> IVGGTDATLGEFPYQLSFQETFIGFSF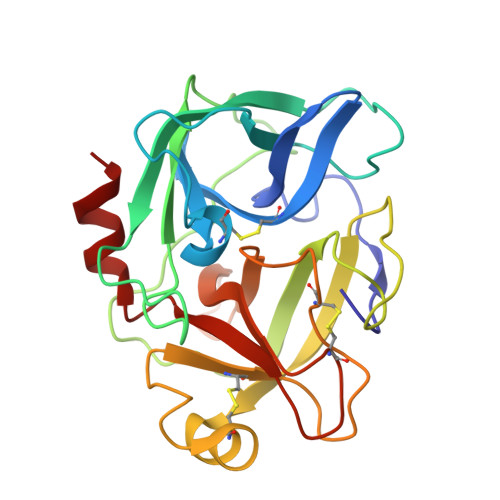HFCGASIYNENYAITAGHCVYGDDYENPSGLQIVAGELDMSVNEGSEQIITVSKIILHENFDYNLLDNDISLLKLSGSLTFNDNVAPIALPEQGHTATGDVIVTGWGTTSEGGNTPDVLQKVTVPLVSDEDCRADYGADEILDSMICAGVPEGGKDSCQGDSGGPLAASDTGSTYLAGIVSWGYGCARPGYPGVYTEVSYHVDWIKANAV> LTATVDGIIQPMLKAYRIPGMAVAVLKDGKAHYFNYGVANRESGQRVSEQTLFEIGSVSKTLTATLGAYAAVKGGFELDDKVSQHAPWLKGSAFDGVTMAELATYSAGGLPLQFPDEVDSNDKMQTYYRSWSPVYPAGTHRQYSNPSIGLFGHLAANSLGQPFEQLMSQTLLPKLGLHHTYIQVPESAMANYAYGYSKEDKPI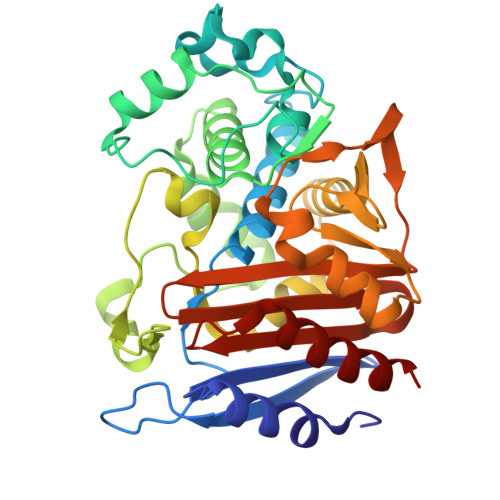RATPGVLAAEAYGIKTGSADLLKFVEANMGYQGDAALKSAIALTHTGFHSVGEMTQGLGWESYDYPVTEQVLLAGNSPAVSFQANPVTRFAVPKAMGEQRLYNKTGSTGGFGAYVAFVPARGIAIVMLANRNYPIEARVKAAHAILSQLAE> MNSQNSQIQPQARYILPSFIEHSSFGVKESNPYNKLFEERIIFLGVQVDDASANDIMAQLLVLESLDPDRDITMYINSPGGGFTSLMAIYDTMQYVRADIQTVCLGQAASAAAVLLAAGTPGKRMALPNARVLIHQPSLSGVIQGQFSDLEIQAAEIERMRTLMETTLARHTGKDAGVIRKDTDRDKILTAEEAKDYGIIDTVLEYRKL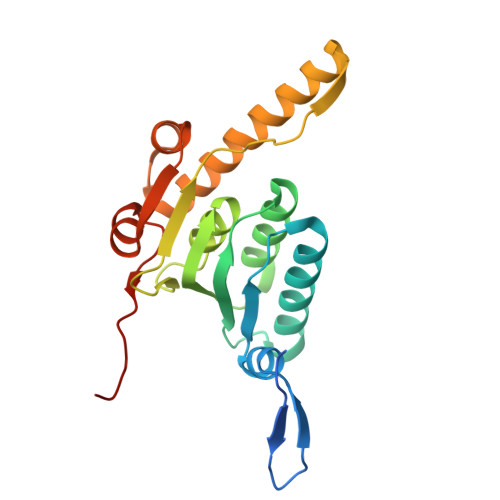SAQTA> SMGKLSEQLKHCNGILKELLSKKHAAYAWPFYK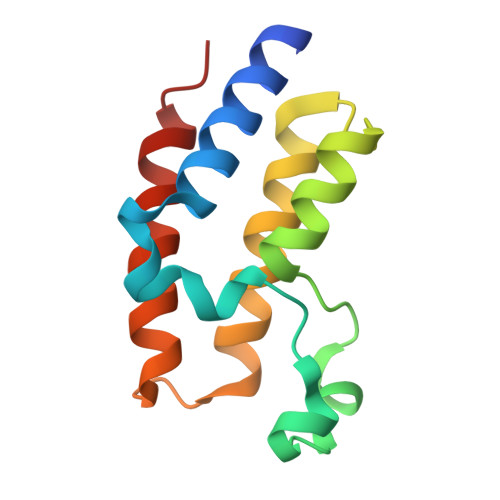PVDASALGLHDYHDIIKHPMDLSTVKRKMENRDYRDAQEFAADVRLMFSNCYKYNPPDHDVVAMARKLHDVFEFRYAKMPD Among these factors, proliferating cell nuclear antigen (PCNA) forms a trimeric ring (sliding clamp) around DNA and directly enhances the activity of proteins involved in replication. Several enzymes bind to PCNA via the PCNA-interacting peptide-box (PIP-box) motif, including DNA-dependent DNA polymerases, flap endonucleases and DNA ligases involved in DNA replication. Analysis of the A. pernix genome showed that the sequence contains three PCNA genes: ApePCNA1 (APE_0162), ApePCNA2 (APE_0441.1) and ApePCNA3 (APE_2182) in the KEGG database. The sliding clamp of A. pernix forms heterotrimers and enhances polymerase activity in the ApePCNA1–ApePCNA2–ApePCNA3 and ApePCNA2–ApePCNA3 complexes.

The crystal structure contains a single ApePCNA1 subunit within the asymmetric unit. The crystals did not contain a threefold axis and the subunits did not form a ring-shaped trimeric structure. The ApePCNA1 subunit is composed of N- and C-terminal domains and a long loop called the inter-domain-connecting loop (IDCL) that connects the two domains formed by Leu130–Gln145. The PCNA rings from other species have an inward α-helix region. The positive surface charge of the α-helix region suggests that ApePCNA1 has an α-helix region located in the inner part of the ring that interacts with the negative charge of the DNA double helix like that in other species. In general, the C-terminal side of the sliding clamp is considered to be the direction of DNA replication, and a group of enzymes responsible for DNA replication bind to the binding pocket near the IDCL. Interestingly, the N-terminus of ApePCNA1 interacted with the cleavage groove of the adjacent ApePCNA1 molecule. In this interaction, the carboxyl group of the N-terminal Asp8 is connected to Arg57 of the neighboring subunit by a hydrogen bond. The hydrophobic side chain of Leu7 is placed in a hydrophobic pocket formed by Met53, Leu60, Pro137, Pro241, Leu257 and Ala259 in an adjacent subunit. The consensus sequence of the PIP-box is QXXhXXaa, where X is any amino acid, h is a hydrophobic amino acid and a is an aromatic amino acid. The 4-EATLDSEF-11 sequence in the N-terminal region of ApePCNA1 is similar to the consensus sequence of the PIP-box. Furthermore, the N-terminal region of ApePCNA1 was suggested to be an anchor sequence that induces PIP-box binding. These results suggest that ApePCNA1 has an unknown function mediated by an N-terminal anchor sequence that results in PIP-box-like interactions.

> MSSEATLDSEFTDYKAMFRYEAKVFKELVDSVSKILDEGLFIITGEGLRLRGMDPARVALVDIEIPSSSFFDFYMAGDVERVELGVNMETLKGVVARAKKGDQLEVRVREDKVLFIVESVVLRRYLLPNLEVIVDVPEDISLEFDATATVIADVVKKTLRDVELVGDIVEFDAGEDYLSIRSVGPERRRVETRLTRESPALIDLEVKEPATSRYDVGYLKRMLGVAKIAESIELSFSTDKPLKMVFKSPDGSRVTYLLAPSTG>GSNGKLRQWLIDQIDSGKYPGLVWENEEKSIFRIPWKHAGRQDYNREEDAALFKAWALFKGKFREGIDKPDPPTWKTRLRCALNKS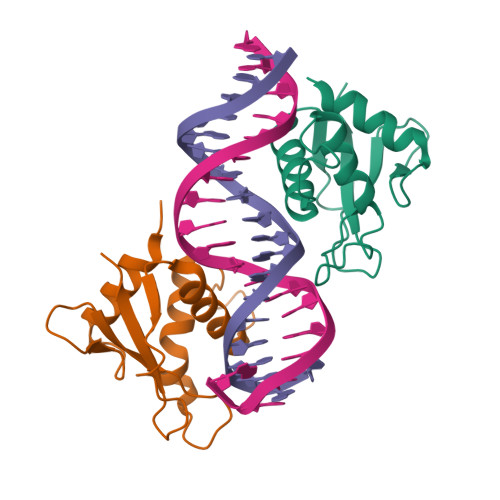NDFEELVERSQLDISDPYKVYRIVP[4x]>MRSNSQGLSLTDSVYERLLSERIIFLGSEVNDEIANRLCAQILLLAAEDASKDISLYINSPGGSISAGMAIYDTMVLAPCDIATYAMGMAASMGEFLLAAGTKGKRYALPHARILMHQPLGGVTGSAADIAIQAEQFAVIKKEMFRLNAEFTGQPIERIEADSDR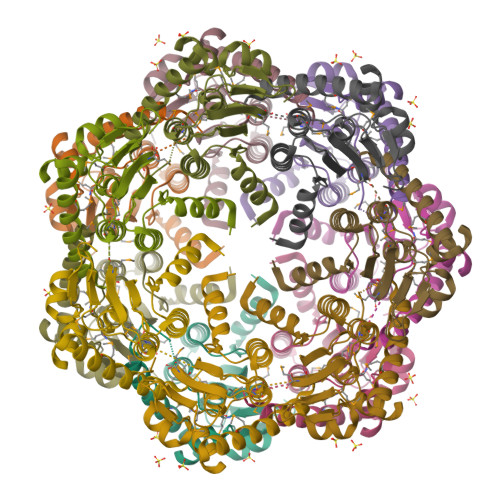DRWFTAAEALEYGFVDHIITRAHVNGEAQ[7x]> MSDVAETLDPLRLPLQGERLIEASAGTGKTFTIAALYLRLLLGLGGSAAFPRPLTVEELLVVTFTEAATAELRGRIRSNIHELRIACLRETTDNPLYERLLEEIDDKAQAAQWLLLAERQMDEAAVFTIHGFCQRMLNLNAFESGMLFEQQLIEDESLLRYQACADFWRRHCYPLPREIAQVVFETWKGPQALLRDINRYLQGEAPVIKAPPPDDETLASRHAQIVARIDTVKQQWRDAVGELDALIESSGIDRRKFNRSNQAKWIDKISAWAEEETNSYQLPESLEKFSQRFLEDRTKAGGETPRHPLFEAIDQLLAEPLSIRDLVITRALAEIRETVAREKRRRGELGFDDMLSRLDSALRSESGEVLAAAIRTRFPVAMIDEFQDTDPQQYRIFRRIWHHQPETALLLIGDPKQAIYAFRGADIFTYMKARSE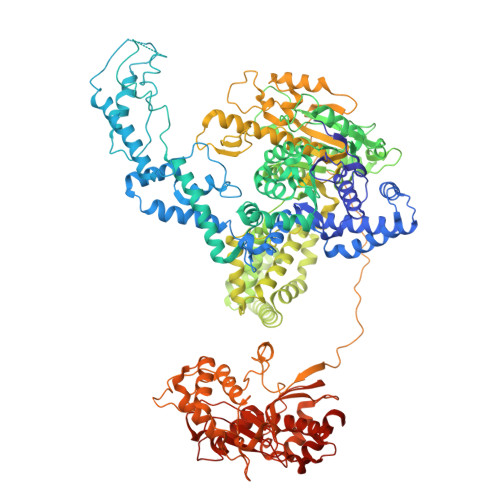VHAHYTLDTNWRSAPGMVNSVNKLFSQTDDAFMFREIPFIPVKSAGKNQALRFVFKGETQPAMKMWLMEGESCGVGDYQSTMAQVCAAQIRDWLQAGQRGEALLMNGDDARPVRASDISVLVRSRQEAAQVRDALTLLEIPSVYLSNRDSVFETLEAQEMLWLLQAVMTPERENTLRSALATSMMGLNALDIETLNNDEHAWDVVVEEFDGYRQIWRKRGVMPMLRALMSARNIAENLLATAGGERRLTDILHISELLQEAGTQLESEHALVRWLSQHILEPDSNASSQQMRLESDKHLVQIVTIHKSKGLEYPLVWLPFITNFRVQEQAFYHDRHSFEAVLDLNAAPESVDLAEAERLAEDLRLLYVALTRSVWHCSLGVAPLVRRRGDKKGDTDVHQSALGRLLQKGEPQDAAGLRTCIEALCDDDIAWQTAQTGDNQPWQVNDVSTAELNAKTLQRLPGDNWRVTSYSGLQQRGHGIAQDLMPRLDVDAAGVASVVEEPTLTPHQFPRGASPGTFLHSLFEDLDFTQPVDPNWVREKLELGGFESQWEPVLTEWITAVLQAPLNETGVSLSQLSARNKQVEMEFYLPISEPLIASQLDTLIRQFDPLSAGCPPLEFMQVRGMLKGFIDLVFRHEGRYYLLDYKSNWLGEDSSAYTQQAMAAAMQAHRYDLQYQLYTLALHRYLRHRIADYDYEHHFGGVIYLFLRGVDKEHPQQGIYTTRPNAGLIALMDEMFAGMTLEEA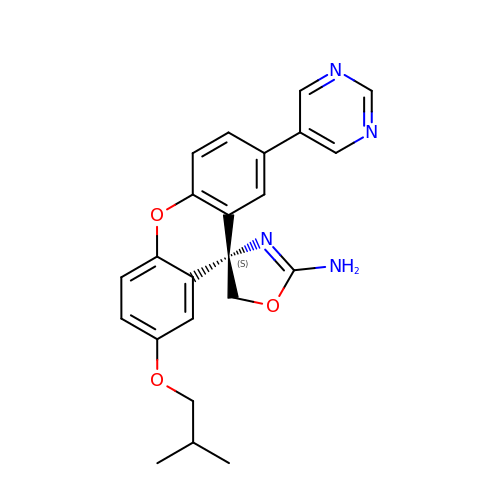(4S)-2'-(2-methylpropoxy)-7'-(pyrimidin-5-yl)spiro[1,3-oxazole-4,9'-xanthen]-2-amine | C23 H22 N4 O3 | JWSHQJYDXNPIKG-QHCPKHFHSA-N>LLQKRVIVSNKREKVINDRRSRQQTVTPAGSEMRYEASFRPENGGLEVVFRLDAPQYHALSVGDRGMLSYKGTAFVAFTPDPL[1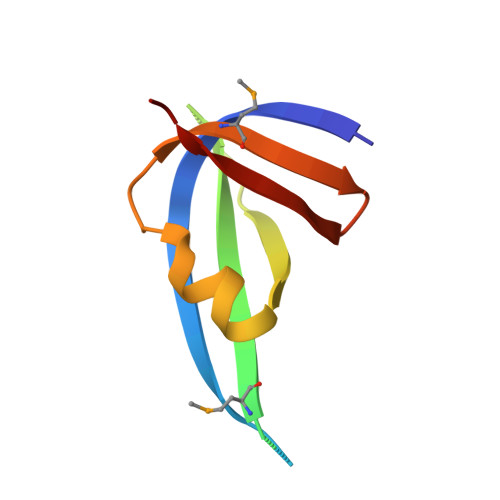6x]>LHSVYQSVELPETHQMLRQTCRDFAEKELVPIAAQLDKEHLFPTSQVKKMGELGLLAMDVPEELSGAGLDYLAYSIALEEISRGCASTGVIMSVNNSLYLGPILKFGSSQQKQQWITPFTNGDKIGCFALSEPGNGSDAGAASTTAREEGDSWVLNGTKAWITNSWEASATVVFASTDRSRQNKGISAFLVPMPTPGLTLGKKEDKLGIRASSTANLIFEDCRIPKENLLGEPGMGFKIAMQTLDMGRIGIASQALGIAQASLDCAVKYAENRHAFGAPLTKLQNIQFKLADMALALESARLLTWRAAMLKDNKKPFTKESAMAKLAASEAATAISHQAIQILGGMGYVTEMPAERYYRDARITEIYEGTSEIQRLVIAG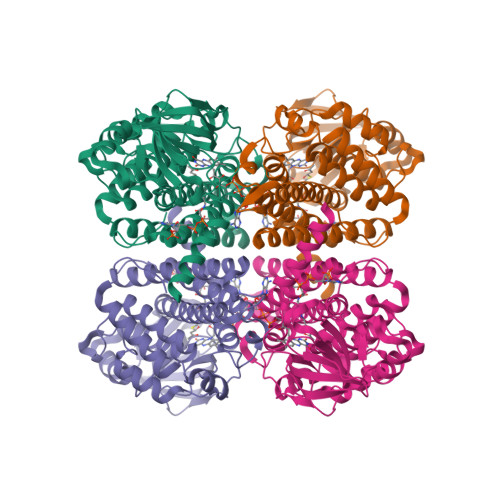HLLRSYRS[2x]> IFGIDDLIIGVLFVAIVETGIGGYLLGSRKESGGGVTKESAEKGFEKIGNDIQILKSSINIAIEKLNDRISHDEQAIRDLTLEIENARSEALLGELGIIRALLVGNIS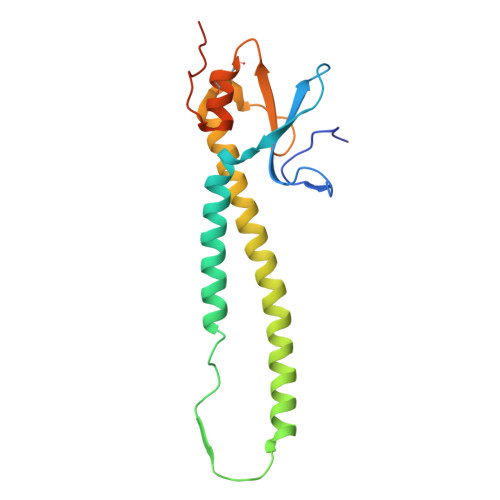IGLQESLWELASEITNRAGDLAVEVSPGCWIIDNNICDQSCQNFIFKFNETAPVPTIPPLDTKIDLQ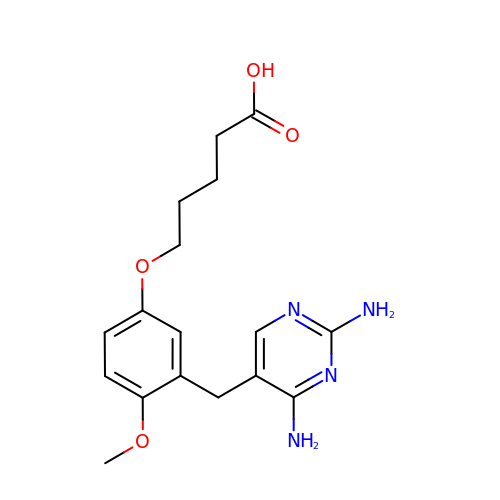2,4-DIAMINO-5-[2-METHOXY-5-(4-CARBOXYBUTYLOXY)BENZYL]PYRIMIDINE | C17 H22 N4 O4 | ALDCXILJAYAUTH-UHFFFAOYSA-N>[2x]MAKKEKKRLQVVISEEQDALLT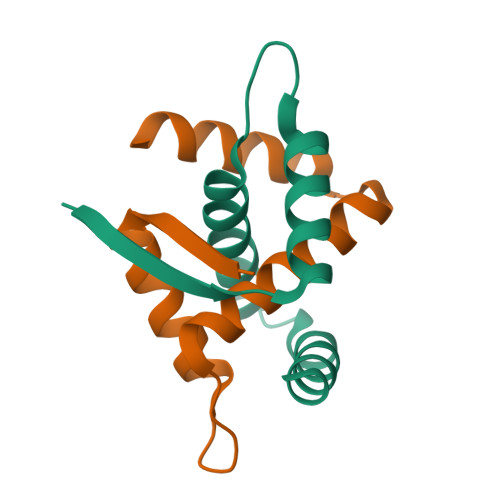RAAYALSSPERAVSKSEVVRLAIEKIARELEEGKAKEELEALLKHLKAEEGEEEA Acinetobacter baumannii produces the catecholate siderophore acinetobactin to scavenge iron, a nutrient essential for several metabolic processes. The biosynthesis begins with BasE, a standalone adenylation domain, which activates and loads 2,3-dihydroxybenzoic acid (DHB) to the phosphopantetheinyl arm of the PCP domain of BasF. Adenylation domains have two subdomains, a large N-terminal subdomain (Acore) and a smaller C-terminal subdomain (Asub), which is highly dynamic, adopting unique conformations to carry out each individual step of the adenylation reaction. Several binding pocket residues were identified within 5 Å of the ligand, including Asn242, Phe243, Ser247, Val336, Val344, and Tyr346.

The V336G mutation further expands the binding pocket, showing improved activity for both 4-fluorosalicylic acid (∼9 fold) and 4-methylsalicylic acid (∼89 fold). This mutant also had significantly higher apparent kcat/KM for 4-azidosalicylic acid (∼40 fold), a trend that was not observed for several of our other mutants. Although the V336G BasE enzyme was soaked with 4-azidosalicylic acid, weak density was observed for the azido group of this molecule. As the azido group may be flexibly positioned or has the potential to hydrolyze to an amino group, possibly promoted by the reducing agent tris(2-carboxyethyl)phosphine (TCEP), we placed 4-aminosalicylic acid in the observed density, which fit well. We docked the 4-azidosalicylic acid molecule into our V336G structure, which showed that the ligand has the potential to bind similarly as our expected pose, with the azido group pointing toward the V336G mutation. The binding pocket of V366G showed an even larger expansion, which provided further space for the azido group of 4-azidosalicylic acid, resulting in the near 40-fold improvement in activity compared to the V336A mutant. When comparing V336G structure to the other BasE structures, we also observed the nearby Tyr346 to slightly turn toward Gly336 as a result of the extra space being present. However, the conformations of the remaining binding pocket residues were maintained. The V336A mutant bound to 4-methylsalicylic acid and the V336G mutant bound to 4-aminosalicylic acid were used to compare with the binding pocket volume of the WT enzyme.

>[2x]MGSSHHHHHSSGENLYFQGHMKKQLIEFVRWSPERAQHYRNKGYWIDQPLTRILTVGVQSHPHSLAIICGERQLSYIELDRLSTNLATRLAEKGLGKGDTALVQLPNVAEFYIVFFALLKAGVVVLNALYSHRQYELNAFIKQIQPKLLIGSRQHEVFSNNQFIDSLHDVNLSPEIILMLNHQATDFGLLDWIETPAETFVDFSSTPADEVAFFQLSGGSTGTPKLIPRTHNDYDYSVRASAEICGLNSNTRLLCALPAPHNFMLSSPGALGVLHAGGCVVMAPNPEPLNCFSIIQRHQVNMASLVPSAVIMWLEKAAQYKDQIQSLKLLQVGGASFPESLARQVPEVLNCKLQQGFGMAEGLVNYTRLDDSDEQIFTTQGRPISSDDEIKIVDEQYREVPEGEIGMLATRGPYTFCGYYQSPEHNSQVFDEDNYYYSGDLVQRTPDGNLRVVGRIKDQINRGGEKIASEEIEKLILLHPEVMHAALVAIVDEQFGEKSCAFIVSRNPELKAVVLRRHLMELGIAQYKLPDQIKLIESLPLTAVGKVDKKQLRSILNTSTTS> YSDDKPFLCTAPGCGRRFTNEDHLAVHKRKHEMTLK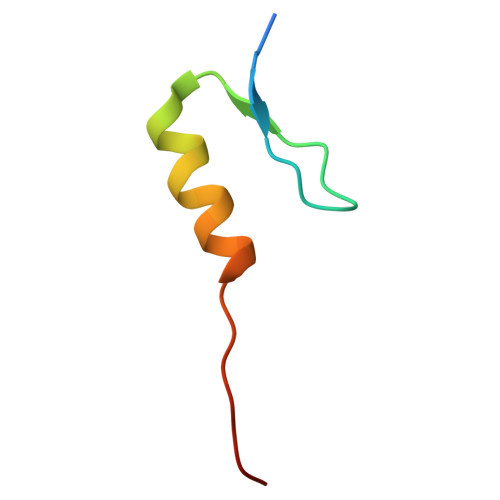FGPA>[2x]MTVDANAASSTTTTTDYYFDSYSHYGIHMEMLKDCHRTTSYRDAMWRNAYLFKDKVVLDVGCGTGILSMFAAKAGARKVIGVDCSTVAVQAREIVKDNGFEDVITIIQGKVEEIQLDEKVDIIISEWMGYFLLYESMLNTVLCARDNLGTPDVKMFPDKANMHVCGITDEQYIQERFNIWDNVQGIDFSYFKRLSFIEPLVDTVERSQIVTNVAPLVSFDINTVKEADLSFTSEFALEAQASRGKRNGGNSIIYVHALSVHFDTPFTAGHEVVILDTTPYSPPTHWRQTVLYLFNPLRMRAGERATFRMKCSPNALNGRDLDISLHVDFEGALQISHYDQDFRLR;>MGMSPKKNSASRPSNNGGGGKTGGGNGNVSHRTDNEQSGNNLSERIIANESLLATESERHATSKSLYGDCTARI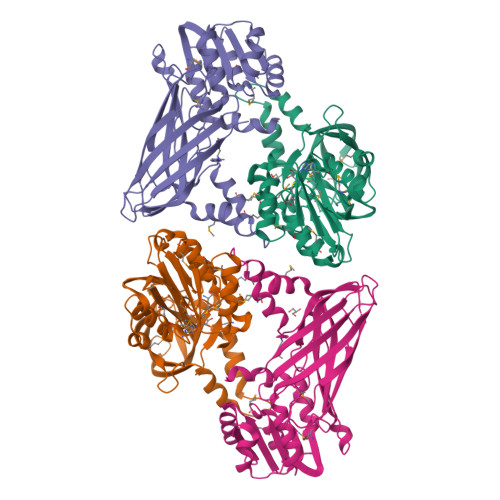SGNLSCIHDRVRLRAYESVLRSIKGKSVLHLGCGMGLVSMIAARSLASAVVAVDRSAIVDAAQVVANKNGLNNISFFRGALVDVVQNFPVRQFDVIICEWMGPFLINDPLLEEALYARNNLLASNGVMCPDSSSIHVVGVSDYCFHMDTVEFWGNVYGFKMEPMKALVQREVEMCRVPTSSIVTTTCLAHTVNIASINNLDDKSSLNDFVVPFSVRATKDTTVNFLTFYIDARFTNPHDPGANFVLGVRPGGTNPWTETSVALHEPLPLKGGEVLSGELKVCLLNPTRGITTVEVTARTSGNVVNIETKGTYNYQRY[2x]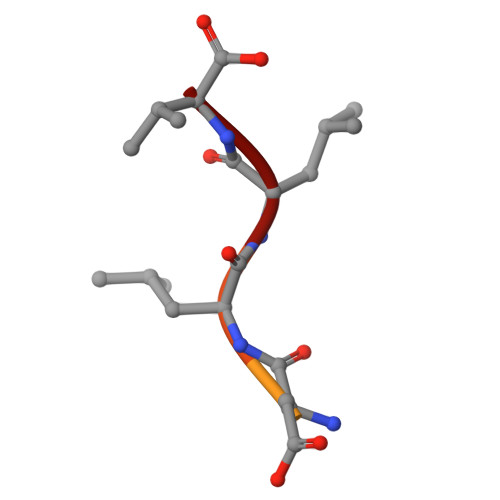> EGVPDLLV>[2x]MQFLQNIPPYLFFTGKGGVGKTSISCATAIRLAEQGKRVLLVSTDPASNVGQVFSQTIGNTIQAIASVPGLSALEIDPQAAAQQYRARIVDPIKGVLPDDVVSSINEQLSGACTTEIAAFDEFTGLLTDASLLTRFDHIIFDTAPTGHTIRLLQLPGAWSSFIDSNPEGASCLGPMAGLEKQREQYAYAVEALSDPKRTRLVLVARLQKSTLQEVARTHLELAAIGLKNQYLVINGVLPKTEAANDTLAAAIWEREQEALANLPADLAGLPTDTLFLQPVNMVGVSALSRLLSTQPVASPSSDEYLQQRPDIPSLSALVDDIARNEHGLIMLMGKGGVGKTTMAAAIAVRLADMGFDVHLTTSDPAAHLSMTLNGSLNNLQVSRIDPHEETERYRQHVLETKGKELDEAGKRLLEEDLRSPCTEEIAVFQAFSRVIREAGKR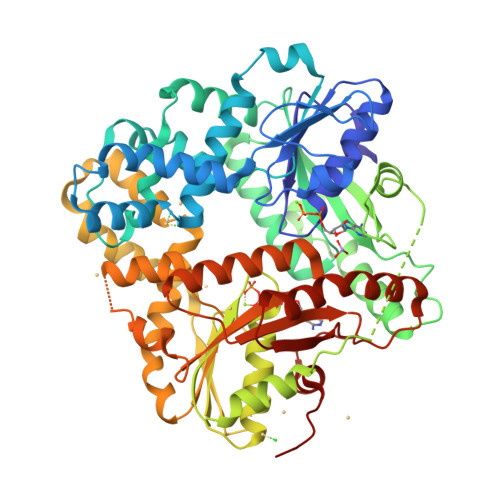FVVMDTAPTGHTLLLLDATGAYHREIAKKMGEKGHFTTPMMLLQDPERTKVLLVTLPETTPVLEAANLQADLERAGIHPWGWIINNSLSIADTRSPLLRMRAQQELPQIESVKRQHASRVALVPVLASEPTGIDKLKQLAGHHHHHH>PVLPQQFVPPTNVRDCIRLRGLPYAATIEDILDFLGEFATDIRTHGVHMVLNHQGRPSGDAFIQMKSADRAFMAAQKCHKKNMKDRYV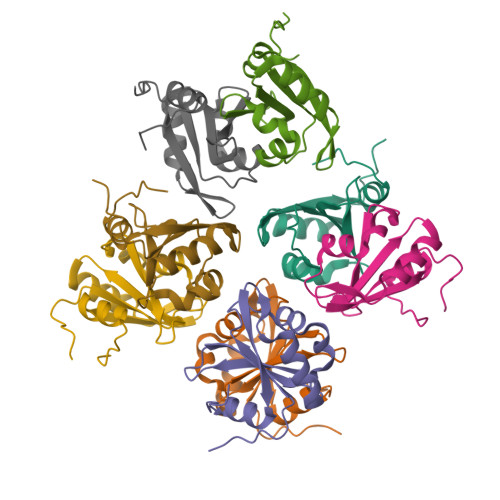EVFQCSAEEMNFVLMGGTLNRN[8x]> TTQKKVVLSSFSIIGDITQNIAKDLVTVTTLVEAGNDSHSYQVTSADAIKIQNADLILCNGLHLEETYMKYFTNLKKGTKIITVTD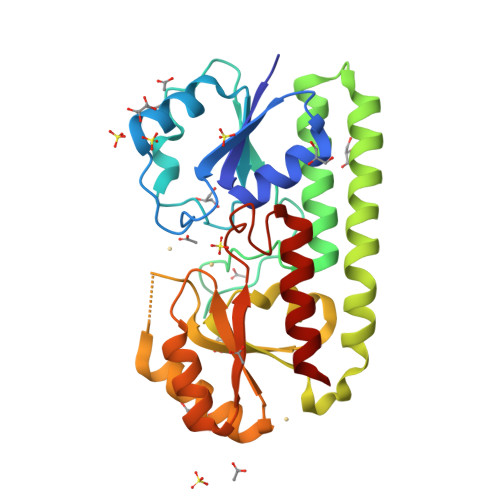GINPIGVSEDTSVDSEPNPHAWMSLTNAMIYIENIRKALTALDPSNAKKYELNAREYSEKIRNSILPLKTRIEKVDPEKRWFVTSEGCLVYLAEDFGFKSLYLWPINSDSERSPSMMRHAINQMRSHKIKFIFSESTNSDQPAKQVAYETNASYGGVLYVDSLSKPDGPAPTYLDLLRFSLTKIVDTLF> EPHSLRYNLTVLSWDGSVQSGFLTEVHLDGQPFLRCDRQKCRAKPQGQWAEDVLGNKTWDRETRDLTGNGKDLRMTLAHIKDQKEGLHSLQEIRVCEIHEDNSTRSSQHFYYDGELFLSQNLETKEWTMPQSSRAQTLAM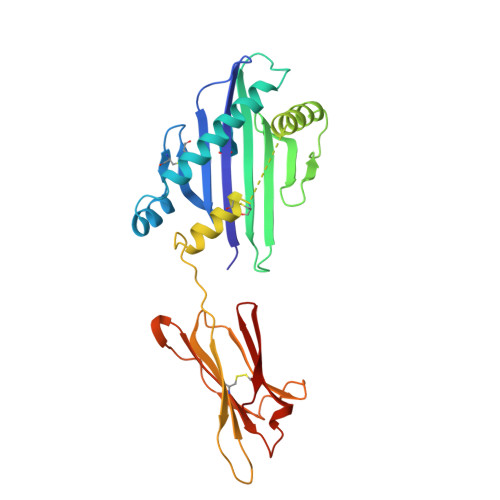NVRNFLKEDAMKTKTHYHAMHADCLQELRRYLKSGVVLRRTVPPMVNVTRSEASEGNITVTCRASGFYPWNITLSWRQDGVSLSHDTQQWGDVLPDGNGTYQTWVATRICQGEEQRFTCYMEHSGNHSTHPVPS>[10x]GLLIKGGVEVLEVKTGVDAITEVECFLNPEMGDPDENLRGFSLKLSAENDFSSDSPERKMLPCYSTARIPLPNLNEDLTSGNLLMWEAVTVQTEVIGITSMLNLHAGSQKVHEHGGGKPIQGSNFHFFAVGGEPLEMQGVLMNYRSKYPDGTITPKNPTAQSQVMNTDHKAYLDKNNAYPVECWVPDPSRNENARYFGTFTGGENVPPVLHVTN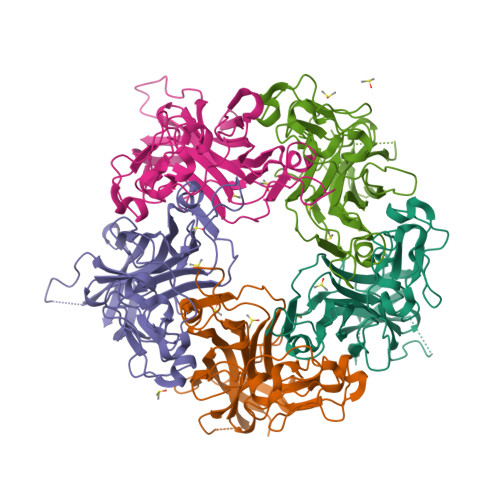TATTVLLDEQGVGPLCKADSLYVSAADICGLFTNSSGTQQWRGLARYFKIRLRKRSVKNPY>[2x]MDIPIPTRQLFINGDWKAPVLNKRIPVINPATQNIIGDIPAATKEDVDVAVAAAKTALTRNKGADWATASGAVRARYLRAIAAKVTEKKPELAKLESIDCGKPLDEAAWDIDDVAGCFEYYADLAEKLDA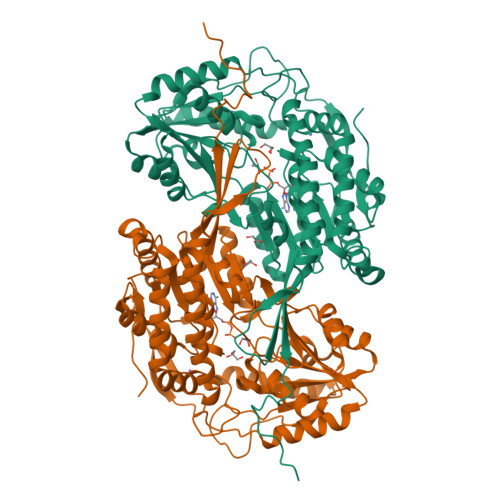RQKAPVSLPMDTFKSHVLREPIGVVGLITPWNYPMLMATWKVAPALAAGCAAILKPSELASLTCLELGEICKEVGLPPGVLNILTGLGPEAGAPLATHPDVDKVAFTGSSATGSKIMTAAAQLVKPVSLELGGKSPLVVFEDVDLDKAAEWAIFGCFWTNGQICSATSRLILHESIATEFLNRIVKWIKNIKISDPLEEGCRLGPVVSEGQYEKILKFVSNAKSEGATILTGGSRPEHLKKGFFIEPTIITDVTTNMQIWREEVFGPVLCVKTFSTEEEAIDLANDTVYGLGAAVISNDLERCERVTKAFKAGIVWVNCSQPCFTQAPWGGVKRSGFGRELGEWGLDNYLSVKQVTQYISEEPWGWYQPPAKL>[2x]AALPDQSFLWNVFQRVDKDRSGVISDTELQQALSNGTWTPFNPVTVRSIISMFDRENKAGVNFSEFTGVWKYITDWQNVFRTYDRDNSGMIDKNELKQALSGFGYRLSDQFHDILIRKFDRQGRGQIAFDDFIQGCIVLQRLTDIFRRYDTDQDGWIQVSYEQYLSMVFSIV;>[2x]NPPPPGFIMHGN

ALG-2 (apoptosis-linked gene 2, gene name: PDCD6), a 22-kDa Ca2+-binding protein, contains five serially-repeated EF-hand motifs (EF1 to EF5) and belongs to the penta-EF-hand (PEF) protein family, including typical calpains, sorcin, grancalcin and peflin (see [1] for a review). ALG-2 binds one of the two mammalian isoforms encoded by different genes, designated Sec31A, in a Ca2+-dependent manner and is recruited to the ER exit sites. ALG-2 binds Ca2+-dependently to a variety of cellular proteins, most of which contain Pro-rich regions, and binding motifs are classified into type 1 (PPYPXnYP) and type 2 (PXPGF). Sec31, conserved from yeast to humans, is a component of the outer layer coat protein complex II (COPII) and is enriched in the endoplasmic reticulum (ER) exit sites, from which cargoes contained in COPII vesicles are transported from the ER to the Golgi apparatus.

The co-crystals of des3-20ALG-2/Sec31A 837–848 obtained in the presence of Zn2+ belonged to space group P64, and the crystals were twinned. The crystal structure was resolved at 2.4 Å resolution. An asymmetric unit of the crystal contained two ALG-2 molecules (chains A and B) as a dimer and two Sec31A peptides (NPPPPGFIMHGN, chains C and D). Three Zn atoms (yellow spheres) are found in the Ca2+-coordinating sites in EF1, EF3 and EF5, essentially and two additional Zn atoms (cyan spheres) are found in the vicinities of EF3 and the Sec31A peptide in each chain. The clustered Pro residues (2PPPP5) form left-handed type II polyproline (PPII) helices. The peptide ligand binds to a hydrophobic pocket designated Pocket 3, which is separated from the ALIX-binding pockets, named Pocket 1 and Pocket 2 (pink and yellow surfaces). Pocket 3 (orange) is formed by residues that are present in EF1 (F27, V31, V35, L48, A51), the EF1–EF2-connecting loop (L52, S53, G55, W57), EF2 (F85, V88, W89, I92), EF3 (T93, Q96, F99, G108, M109) and EF4 (F148). Several Pocket 3-forming residues interact with the Sec31A peptide at the side chain or main chain carbon atoms of the peptide by hydrophobic interactions (common contact residues in both chains B and D are indicated in bold face: A51, L52, S53, W57, F85, W89, I92, F148). Hydrogen bonds are formed between chains A and C (S53OG/P3O, S53O/G6N, S53N/G6O, A51O/I8N) and between chains B and D (S53OG/P3O, S53N/G6O, A51O/I8N). The Sec31A peptide binds ALG-2 at a hydrophobic pocket, designated Pocket 3, formed by residues that are present from EF1 to EF3, except for F148 (the loop in EF4). This pocket is completely separated from Pockets 1 and 2, which are formed by residues from EF2 to EF5.A non-turreted virus consisting of a 12-segment dsRNA genome, mud crab reovirus (MCRV), which may belong to a new order of Reovirales, infects the economically important crab Scylla serrata. Like other members of Reovirales, MCRV packages its dsRNA segments and a number of RNA-dependent RNA polymerase (RdRp) inside a double-layered icosahedral capsid. Using cryo-EM, we determined the structure of mud crab reovirus (MCRV), a 12-segmented dsRNA virus that is a putative member of Reovirales in the non-turreted Sedoreoviridae family, to near-atomic resolutions with icosahedral symmetry (3.1 Å) and without imposing icosahedral symmetry (3.4 Å). These structures revealed the organization of the major capsid proteins in two layers: an outer T = 13 layer consisting of VP12 trimers and unique VP11 clamps, and an inner T = 1 layer consisting of VP3 dimers.

The three-dimensional structure of the qMCRV was first determined to 3.1 Å resolution with icosahedral symmetry. The map clearly shows an outer and inner capsid layer; the inner capsid layer is a thin shell composed of 60 copies of a VP3 dimer, while the outer capsid, arranged on a T = 13 lattice, is thicker and composed of VP12 trimers organized in a similar way to the previously reported low-resolution reconstruction. Interdigitating these trimers are two smaller densities per asymmetric unit and assigned to be VP11. A VP3 dimer, containing two chemically identical subunits (A and B) with slightly different conformations in an asymmetric unit, forms the thin inner shell of the MCRV. In context, the five N-terminal arms of VP3B form a “belt” around the five-fold vertex that function to link and stabilize the pentamer of VP3 dimers. VP12, the primary outer shell trimer protein, is comprised of a β-sandwich (two β-sheets of four antiparallel strands) atop an all α-helical base. Two VP11 subunits per asymmetric unit are embedded between VP12 trimers and bridge multiple asymmetric units. One of the two VP11 subunits (VP11A) bridges the adjacent asymmetric units around the same 5-fold vertex and block the narrow opening, previously denoted as a type II channel, while the other (VP11B) is located along the icosahedral 2-fold axis and block the type III channel. A striking feature of MCRV is the large separation in the inner capsid underneath VP11B at the type III channel. VP11B may provide the “missing” interactions to clamp the neighboring VP3 inner capsid proteins that have no direct interactions among different decamers.

>MNWSKAINFQPFMLETRPPLTTIPIMDQLVEIGERSNQKWSMTDRLFFAIRKINPIFVTSSQIPSKFDYTILQMPTQLIASLKETLLFLAFSYYLREYQDKVGQMKFYPVAMKNMIPIVNYLKDRVHNNFDTTLEQAYRQNVVHTLSASDAFDLLSGMIATTRLDLIQRTRICPELLNVLNKMSFILIYAPNRPSILSWKNQS[2x];>[2x]MASTTRLVNDRKQLEQQVKDDARILADARGLNITTVANDSATGGQAIRNVGPNDEATIKALDNVIKQIEALSVIVNRSEKADDAQILGPNTYKQLLEHLFSPEENVYILLPIQAYTGGVIDRRDASFSNFAYSIASKLMMELSAATHNKIFTDYTRIAASALGPEISTEGMPLFSLIESLELTEAETSRLPVIQDSMVIQKSTATVGNAQQGISTINIKRVPFVGSAFQQVIDQLLWEYSTTSLTTKEQRRQRITEMVNDRRIMIQKLTLAEKPQVMRHVTTEINNDLFFKMSPVAQLYIYHLDRAFLDGVGFTPLAEKQQQLQLQLKTNILTANLIRSAINGMNTESNLEVAIKMMQAAQLHRASIEIAFPMNVSLSPEIIVQCFIVWMSIPEQLLSDRSNFIIAAVIWAGFSADDSYADIMRRSARASDRQNYDIIKAALSSRKFKLPRASTTLFDENEPVVRRYQIGRVYAPFPVDRYGSPVYSNCTKVELASDYNAEGFTIRKDDFRALQAVLRIDEDRAADMFTTLRIMISSIPAVWYDAEVVHYPHTAVELEQLAAYGLTGAYPRTNHSVDTIVKTVNNISATYSTIAQMLSTIDLDPTRYGTSESIDKFKIAWENVESVLNMEGNDFVKTIMYAYEDNFPKKDFYMMLKQIASDGQGAHPIAAAIDQLRTIVYREPERFGYIDSVILTHNPDVDTAYNRFFHLHPIVTNQPSNTIKNAQLWNEMRLEQQVEHIKAGPVRIIGPFHVTYNYLSEEEDMPATSHIIMKDNMILNDHLTFNFVKRERRNNKKRVSSFRYKAVEMYVAVRISRFQLEVLRDLHDLVRSRTYLDVSKSPLATTPIRVVEYVR;>MNLEINNFAPAISSIGSQLCSLSAQKLLTCRKQYGNGAKSFEEFYAEIGGIIGMMGINSQTPSGIREAIYRLYQSAFLFGDIFPESFGIQNTQNIKPPPGFTAPAKKLEVVLPQGGAFDLIYNNGEIRVTTTRNVQAGDLVCTVTFPIQGSVIATRNCHVNEIGGQLTTTRPEIIASVPMPARTVIVASFDAIEIGYGEGDDLFAIGIAILSNRFNGQITPMSRHNYMTQMFANLPANMSERDSSAVLHFAQAAPVVLGMMERLTGAPKWVLDY[13x]>[4x]VPRGSHMNKICKILNIKYPVIQGGMAWVATASLASAVSNAGGLGIIAAGNAPKEAIKKEIVECKKLTDKPFGVNVMLMSPFVDDIIDLIIEEKVQVITTGAGNPAKYMDRLKEAGTKVIPVVPTIALAQRMEKLGATAVIAEGTEGGGHIGELTTMVLVPQVADAVNIPVIAAGGIVDGRGIAASFALGASAVQVGTRFICSEECSVHSNYKNLVLKAKDRDAIVTGRSTGHPVRTLKNKLSK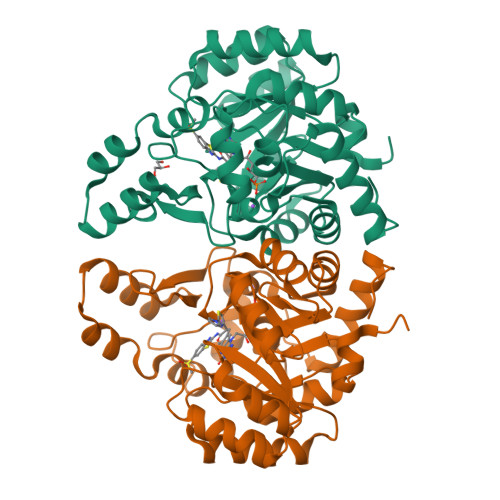EFLKMEQNGATPEELDKKGTGALRFATVDGDIEKGSFMAGQSAAMVKEITPCKEIIEAMVNQAREIMPAIEL>MAVLKIISWNVNGLR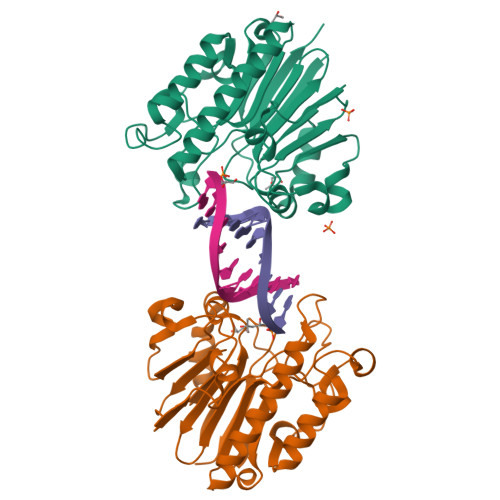AVHRKGFLKWFMEEKPDILCLQEIKAAPEQLPRKLRHVEGYRSFFTPAERKGYSGVAMYTKVPPSSLREGFGVERFDTEGRIQIADFDDFLLYNIYFPNGKMSEERLKYKLEFYDAFLEDVNRERDSGRNVIICGNFNTAHREIDLARPKENSNVSGFLPVERAWIDKFIENGYVDTFRMFNSDPGQYTWWSYRTRARERNVGWRLDYFFVNEEFKGKVKRSWILSDVMGSDHCPIGLEIELLEHHHHHH[2x]>[60x]MWRVCARRAQNAAPRAGFGARWTAFREEPGAPCVTPQAGSALARCSSKTPGYGRVRALCGWSPVSRATPRNRVLLQLWGSPSRRWYSLPPHQKVPLPSLSPTMQAGTIARWEKKEGEKINEGELIAEVETDKATVGFESVEECYMAKILVAEGTRDVPVGAIICITVDKPEDVEAFKNYTLDSSAAPAPPAAPAPTPAAPAPSPTPSAQAPGSSYPTHMQVLLPALSPTMTMGTVQRWEKKVGEKLNEGDLLAEIETDKATIGFEVQEEGYLAKILIPEGTRDVPLGTPLCIIVEKEADIPAFADYRPAEVTDLKPPAPPPIPSPAAPVPPAPQPVAPPPSAPRPAAPAGPKGRVFVSPLAKKLAAEKGIDLTQVKGTGPDGRIIKKDIDSFVPTKAAPTPAAAVPPPSPGVAPVPTGVFTDIPISNIRRVIAQRLMQSKQTIPHYYLSIDVNMGEVLLVRKELNKMLEGKSKISVNDFIIKASALACLKVPEANSSWMDTVIRQNHVVDISVAVSTPAGLITPIVFNAHIKGLETIANDVVSLATKAREGKLQPHEFQGGTFTISNLGMFGIKNFSAIINPPQACILAIGASEDRLVPADNEKGFDVASMMSVTLSCDHRVVDGAVGAQWLAEFRKYLEKPITMLL

The α-keto acid dehydrogenase complex family catalyzes the essential oxidative decarboxylation of α-keto acids to yield acyl-CoA and NADH. PDC, OGDC, and BCKDC are each comprised of multiple copies of a substrate-specific dihydrolipoamide acetyltransferase (E2p), dihydrolipoamide succinyltransferase (E2o), or dihydrolipoamide acyltransferase (E2b) inner catalytic (IC) core surrounded by multiple copies of the respective α-keto acid dehydrogenase (E1p, E1o, or E1b) and universal dihydrolipoamide dehydrogenase (E3) components. Here, we report the cryo-electron microscopy structures of the endogenous cubic 2-oxoglutarate dehydrogenase complex (OGDC) and icosahedral pyruvate dehydrogenase complex (PDC) cores from bovine kidney determined at resolutions of 3.5 Å and 3.8 Å, respectively. In addition, despite sharing a similar monomeric fold, OGDC and PDC E2 cores have distinct interdomain and intertrimer interactions, which suggests a means of modulating self-assembly to mitigate heterologous binding between mismatched E2 species.

The pyruvate dehydrogenase complex (PDC; components suffixed by ‘p’) is an essential element of life that catalyzes the oxidative decarboxylation of pyruvate to acetyl-coenzyme A (acetyl-CoA). We initially identified PDC based on its distinct icosahedral architecture. This is confirmed by atomic model building of the bovine E2p sequence into the icosahedral cryo-EM density map, which showed good agreement between the sequence and the respective side chain densities. For E2p, the backbones of residues 420–647 are fully traceable, except for residues 519 and 520, which lack densities. Due to missing density at the βE–βF β-turn, two residues (Ala519 and Gly520) are unmodelled in our E2p model. Adjacent to the region of missing density, a putative density for the lipoyl moiety was identified near the catalytic residues Ser566 and His620′ and the gatekeeper residue Leu521. In E2p, H2 instead has a length of 14 residues (Gly455–Leu468) and is a single, uninterrupted helix. H7 of E2p (Pro642–Leu646) has a length of five residues and one additional residue (Leu647) at the C-terminus. The E2p knob has one hydrophobic surface that binds a single hydrophobic pocket in the socket. Heterogeneity of E3BP distribution precludes identification and experimental structural determination of E3BP from native mammalian PDC.(TRANS-12,13-EPOXY)-11-HYDROXY-9(Z)-OCTADECENOIC ACID | C18 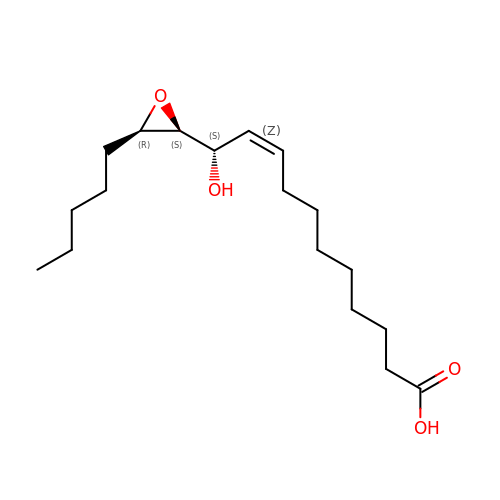H32 O4 | UZCLYICSWADYGM-RXWDXHPSSA-N> GAMGALPPDGHP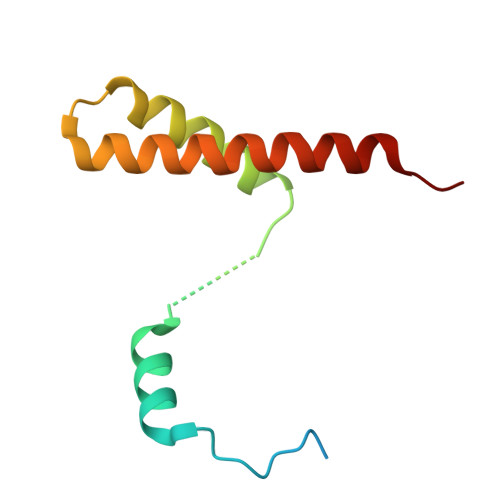VEPHLERLYPTAQSKRSLWDFASPGYTFHGLHRAQDYRRELDTLQSLLTTSQSSELQAAAALLKCQQDDDRLLQIILNLLHKV>MSEPIRVLVTGAAGQIAYS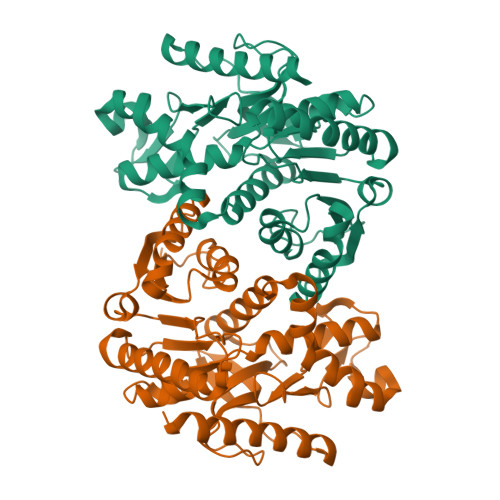LLYSIGNGSVFGKDQPIILVLLDITPMMGVLDGVLMELQDCALPLLKDVIATDKEDVAFKDLDVAILVGSMPRREGMERKDLLKANVKIFKSQGAALDKYAKKSVKVIVVGNPANTNCLTASKSAPSIPKENFSCLTRLDHNRAKAQIALKLGVTANDVKNVIIWGNHSSTQYPDVNHAKVKLQGKEVGVYEALKDDSWLKGEFVTTVQQRGAAVIKARKLSSAMSAAKAICDHVRDIWFGTPEGEFVSMGVISDGNSYGVPDDLLYSFPVVIKNKTWKFVEGLPINDFSREKMDLTAKELTEEKESAFEFLSSA[2x]>[2x]EGLTIDLKNFRKPGEKTFTQRSRLFVGNLPPDITEEEMRKLFEKYGKAGEVFIHKDKGFGFIRLETRTLAEIAKVELDNMPLRGKQLRVRFACHSASLTVRNLPQYVSNELLEEAFSVFGQVERAVVIVDDRGRPSGKGIVEFSGKPAARKALDRCSEGSFLLTTFPRPVTVEPMDQLDDEEGLPEKLVIKN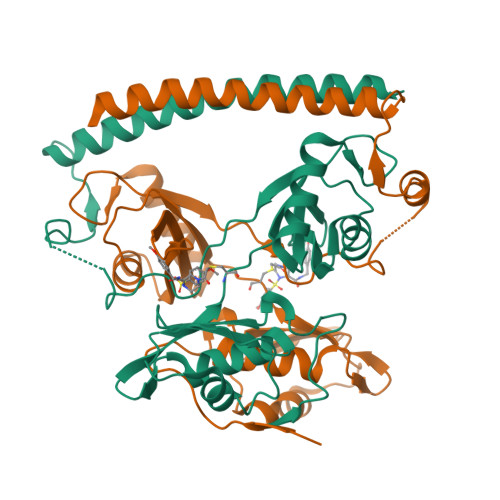QQFHKEREQPPRFAQPGSFEYEYAMRWKALIEMEKQQQDQVDRNIKEAREKLEMEMEAARHEHQVMLM>GSHMVRESSFVEKMKKTGRNIIVFYGSQTGTAEEFANRLSKDAHRYGMRGMSADPEEYDLADLSSLPEIDNALVVFCMATYGEGDPTDNAQDFYDWLQETDVDLSGVKFAVFGLGNKTYEHFNAMGKYVDKRLEQLGAQRIFELGLGDDDGNLEEDFITWREQFWLAVCEHFGVEATGEESSIRQYELVVHTDIDAAKVYMGEMGRLKSYENQKPPFDAKNPFLAAVTTNRKLNQGTERHLMHLELDISDSKIRYESGDHVAVYPANDSALVNQLGKILGADLDVVMSLNNLDEESNKKHPFPCPTSYRTALTYYLDITNPPRTNVLYELAQYASEPSEQELLRKMASSSGEGKELYLSWVVEARRHILAILQDCPSLRPPIDHLCELLPRLQARYYSIASSSKVHPNSVH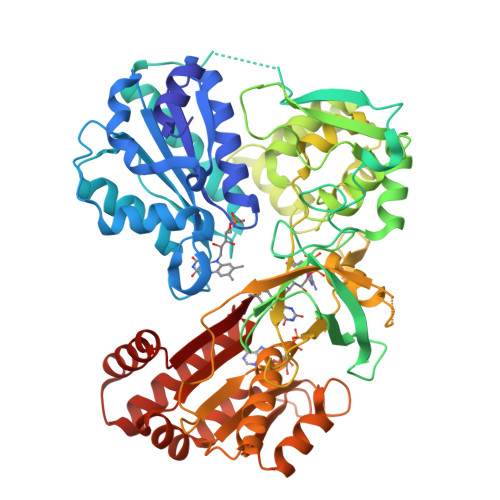ICAVVVEYETKAGRINKGVATNWLRAKEPVGENGGRALVPMFVRKSQFRLPFKATTPVIMVGPGTGVAPFIGFIQERAWLRQQGKEVGETLLYYGCRRSDEDYLYREELAQFHRDGALTQLNVAFSREQSHKVYVQHLLKQDREHLWKLIEGGAHIYVCGDARNMARDVQNTFYDIVAELGAMEHAQAVDYIKKLMTKGRYSLDVWS[2x]> MVFQSHIGVLAFPFGTHAAPLLTVVQRLATSSPHTLFSFFNSAVSNSTLFNNGVLDSYDNIRVYHVWDGTPQGQAFTGSHFEAVGLFLKASPGNFDKVIDEAEVETGLKISCLITDAFLWFGYDLAEKRGVPWLAFWTSAQCALSAHMYTHEILKAVGSNGVGETAEEELIQSLIPGLEMAHLSDLPPEIFFDKNPNPLAITINKMVLKLPKSTAVILNSFEEIDPIITTDLKSKFHHFLNIGPSILSSPTPPPPDDKTGCLAWLDSQTRPKSVVYISFGTVITPPENELAALSEALETCNYPFLWSLNDRAKKSLPTGFLDRTKELGMIVPWAPQPRVLAHRSVGVFVTHCGWNSILESICSGVPL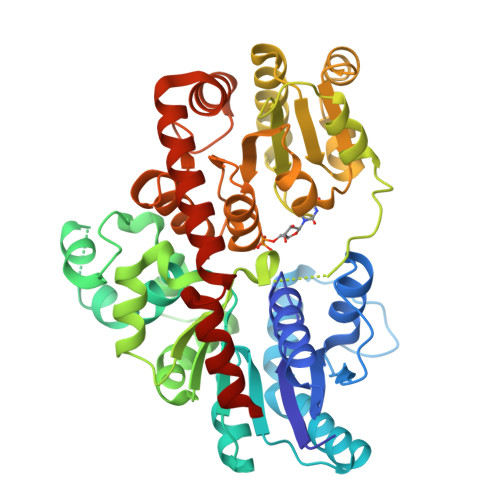ICRPFFGDQKLNSRMVEDSWKIGVRLEGGVLSKTATVEALGRVMMSEEGEIIRENVNEMNEKAKIAVEPKGSSFKNFNKLLEIINAPQSS7-BROMO-1-[2-(DIETHYLAMINO)ETHYL]-5-(2-FLUOROPHENYL)-1,3-DIHYDRO-2H-1,4-BENZODIAZEPIN-2-ONE | C21 H23 Br F N3 O 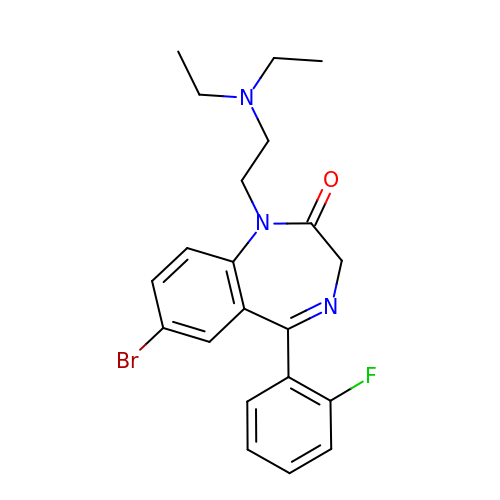| FRXOAXNCRZNTCO-UHFFFAOYSA-N> MTQINLTLVSELADQHLMAEYRELPRVFGAVRKHVANGKRVRDFKISPTFILGAGHVTFFYDKLEFLRKRQIELIAECLKRGFNIKDTTVQDISDIPQEFRGDYIPHEASIAISQARLDEKIA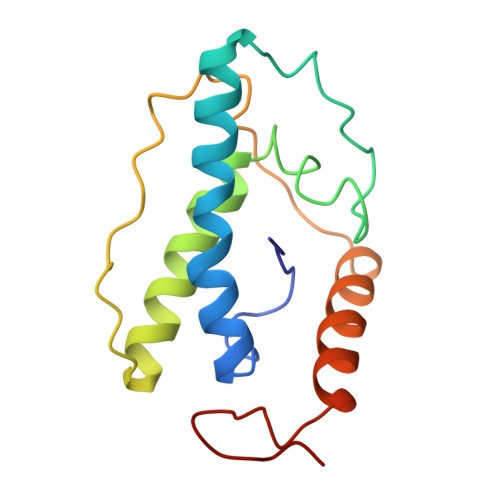QRPTWYKYYGKAIYA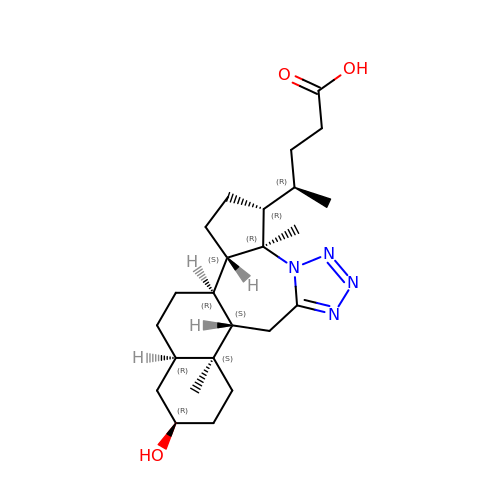(4~{R})-4-[(1~{R},2~{S},5~{R},6~{R},13~{S},14~{S},17~{R},19~{R})-6,14-dimethyl-17-oxidanyl-7,8,9,10-tetrazapentacyclo[11.8.0.0^{2,6}.0^{7,11}.0^{14,19}]henicosa-8,10-dien-5-yl]pentanoic acid | C24 H38 N4 O3 | MIQKAEOABWRKCI-VPUMZWJWSA-N>SEFSRHSEKIAIRDF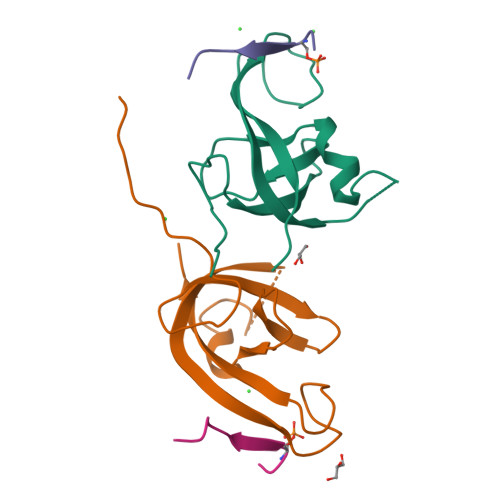QVGDLVLIILDERHDNYVLFTVSPTLYFLHSESLPALDLKPGEGASGASRRPWVLGKVMEKEYCQAKKAQNRFKVPLGTKFYRVKAVSWNKKV[2x];>[2x]SSEDSFVEIRMAE> T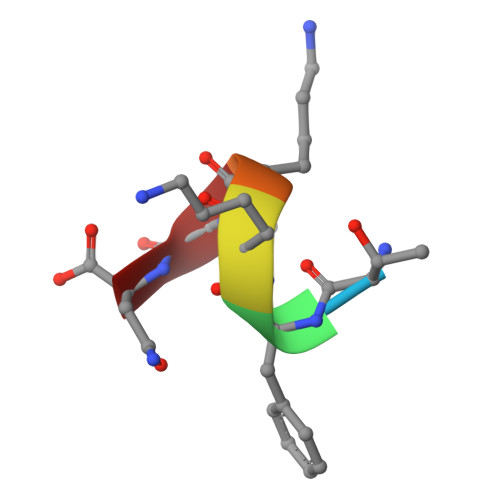FKKTN> GSHMASQVGVIKPWLLLGSQDAAHDLDTLKKNKVTHILNVAY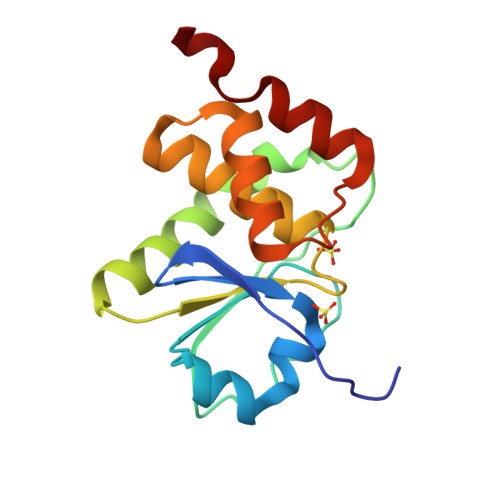GVENAFLSDFTYKSISILDLPETNILSYFPECFEFIEEAKRKDGVVLVHANAGVSRAAAIVIGFLMNSEQTSFTSAFSLVKNARPSICPNSGFMEQLRTYQEGKE methyl [3-(aminomethyl)phenoxy]acetate | C10 H13 N O3 | 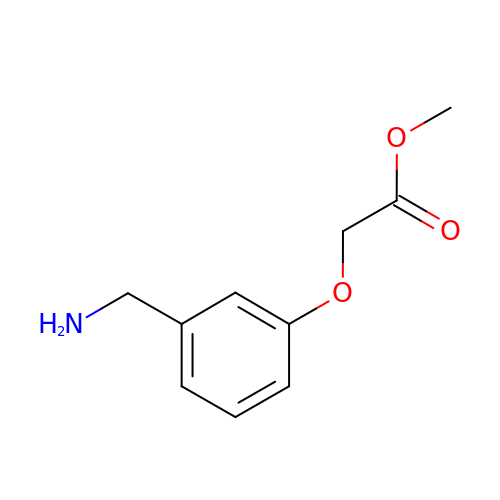HUXMCFLTUUEWMA-UHFFFAOYSA-N>MEFKKVAKETAITLQSYLTYQAVRLISQQLSETNPGQAIWLGEFSKRHPIQESDLYLEAMMLENKELVLRILTVRENLAEGVLEFLPEMVLSQIKQSNGNHRRSLLERLTQVDSSSTDQTEPNPGESDT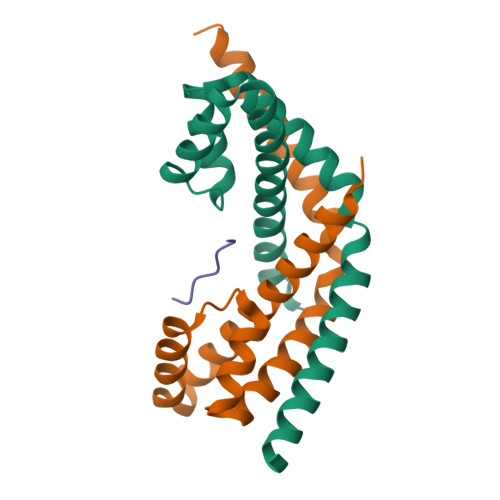SEDSE[6x];> EIKFEFD>[2x]SMADRNLRDLLAPWVPDAPSRALREMTLDSRVAAAGD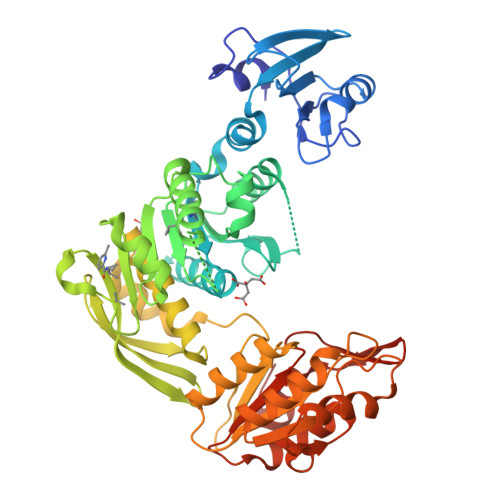LFVAVVGHQADGRRYIPQAIAQGVAAIIAEAKDEATDGEIREMHGVPVIYLSQLNERLSALAGRFYHEPSDNLRLVGVTGTNGKTTTTQLLAQWSQLLGEISAVMGTVGNGLLGKVIPTENTTGSAVDVQHELAGLVDQGATFCAMEVSSHGLVQHRVAALKFAASVFTNLSRDHLDYHGDMEHYEAAKWLLYSEHHCGQAIINADDEVGRRWLAKLPDAVAVSMEDHINPNCHGRWLKATEVNYHDSGATIRFSSSWGDGEIESHLMGAFNVSNLLLALATLLALGYPLADLLKTAARLQPVCGRMEVFTAPGKPTVVVDYAHTPDALEKALQAARLHCAGKLWCVFGCGGDRDKGKRPLMGAIAEEFADVAVVTDDNPRTEEPRAIINDILAGMLDAGHAKVMEGRAEAVTCAVMQAKENDVVLVAGKGHEDYQIVGNQRLDYSDRVTVARLLGVIA>MGNCSTNLSCCANGQKTIVQDKVCIDWTAAATAAIIYADNISQDIYASGYLKVDTGTGPVTIVFYSGGVTGTAVETIVVATGSSASFT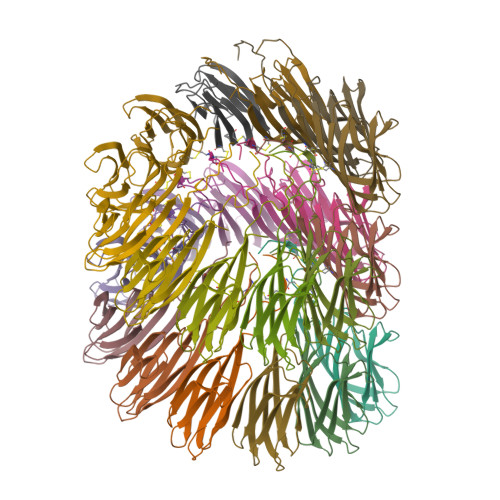VRRFDTVTILGTAAAETGEFCMTIRYTLS[23x]>[2x]NKEYTEEQKQTLEQEQKEFLSQTTTPELEADDGFIVTSESSAQSTPSMSALSGNISPDSQTSDPITKAVRETIIQPQKDNLIEQILKDLAALTDRDLAEQKRKEIEEEKEKDKTLSTFFGNPANREFIDKALEKPELKKKLESIEIAGYKNVHNTFSAASGYPGGFKPVQWENHVSASDLRATVVKNDAGDELCTLNETTVKTKPFTLAKQDGTQVQISSYREIDFPIKLDQAD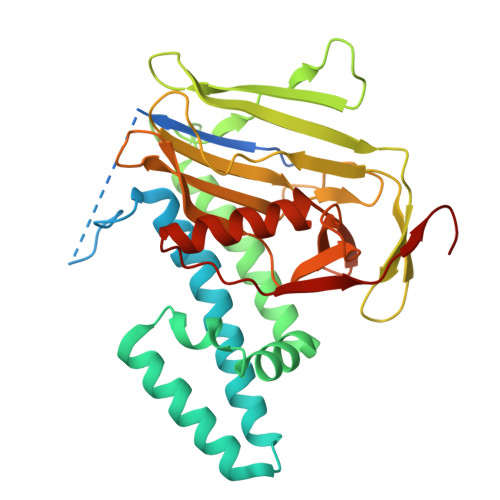GSMHLSMVALKADGTKPSKDKAVYFTAHYEEGPNGKPQLKEISSPKPLKFAGTGDDAIAYIEHGGEIYTLAVTRGKYKEMMKEVELNQGQSVDLSQAEDIIIGQGQ N-[3-[1,1-bis(oxidanylidene)-1,2-thiazolidin-2-yl]-4-chloranyl-phenyl]-2-methoxy-5-methyl-benzenesulfonamide 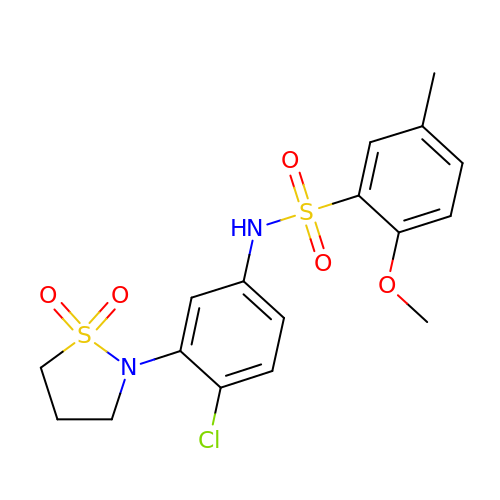| C17 H19 Cl N2 O5 S2 | PNCFQLGARJZZFI-UHFFFAOYSA-N> MFLPPPECPVFEPSWEEFADPFAFIHKIRPIAEQTGICKVRPPPDWQPPFACDVDKLHFTPRIQRLNELEAQTRVRDYTLRTFGEMADAFKSDYFNMPVHMVPTELVEKEFWRLVSTIEEDVTVEYGADIASKEFGSGFPVRDGKIKLSPEEEEYLDSGWNLNNMPVMEQSVLAHITADICGMKLPWLYVGMCFSSFCWHIEDHWSYSINYLHWGEPKTWYGVPGYAAEQLENVMKKLAPELFVSQPDLLHQLVTIMNPNTLMTHEVPVYRTNQCAGEFVITFPRAYHSGFNQGFNFAEAVNFCTVDWLPLGRQCVEHYRLLHRYCVFSHDEMICKMASKADVL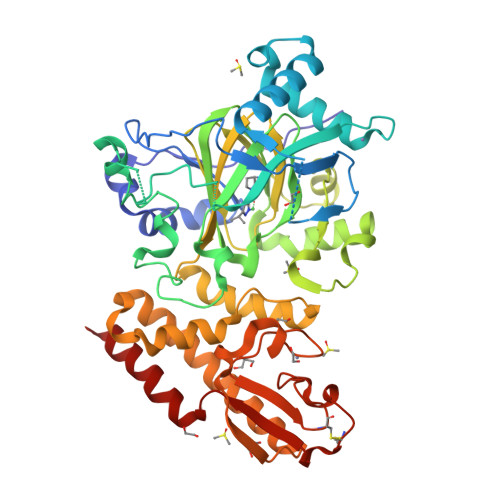DVVVASTVQKDMAIMIEDEKALRETVRKLGVIDSERMDFELLPDDERQCVKCKTTCFMSAISCSCKPGLLVCLHHVKELCSCPPYKYKLRYRYTLDDLYPMMNALKLRAES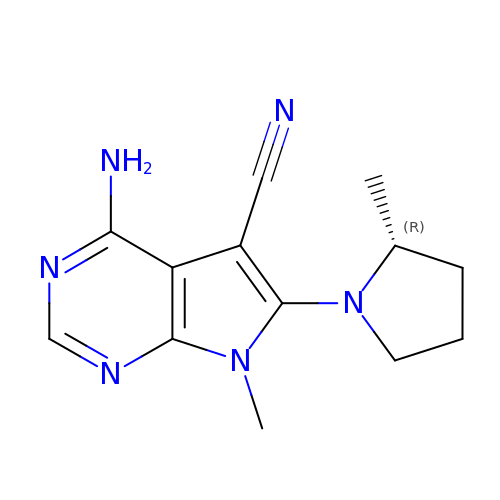4-amino-7-methyl-6-[(2R)-2-methylpyrrolidin-1-yl]-7H-pyrrolo[2,3-d]pyrimidine-5-carbonitrile | C13 H16 N6 | DCOXMFDDEKIJAR-MRVPVSSYSA-N>[4x]GMDSGESGPQQWAGVVKVNDRMGYVTFTDA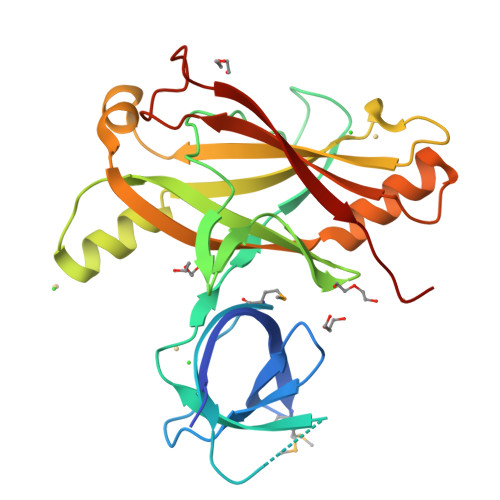AGTELIPTNTIPVTLNARMAYIYCQVDEGQDLSTNPKSIKITLLADPTGIDATAITTPKVGESGDVTTNAPVGSLSFVSGYSTVAPFQFSENTIVLPVLYRVKNVTTTEDIKNELAKHTFTLVCYTDDIKSGDTILKLYLRYKVEDEPAAIAERATRTSSFKAYEISQILREYTLKSGQTKPAKITIVAQQNEYNNKLEDTSTIEKVYEIEYKTAE>MRGSHHHHHHGSMDKNIIIGAMTALITPFKNGKVDEQSYARLIKRQIEN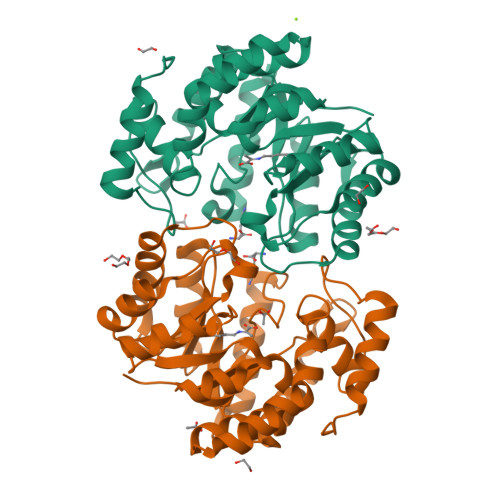GIDAVVPVGTTGESATLTAEEHRTCIEIAVETCKGTKVKVLAGAGSNATHEAVGLAKFAKEHGADGILSVAPYYNKPTQQGLYEHYKAIAQSVDIPVLLYNVPGRTGCEISTDTIIKLFRDCENIYGVKEASGNIDKCVDLLAHEPRMMLISGEDAINYPILSNGGKGVISVTSNLLPDMISALTHFALDENYKEAKKINDELYNINKILFCESNPIPIKTAMYLAGLIESLEFRLPLCSPSKENFAKIEEVMKKYKIKGF[6x]SULFAMIC ACID 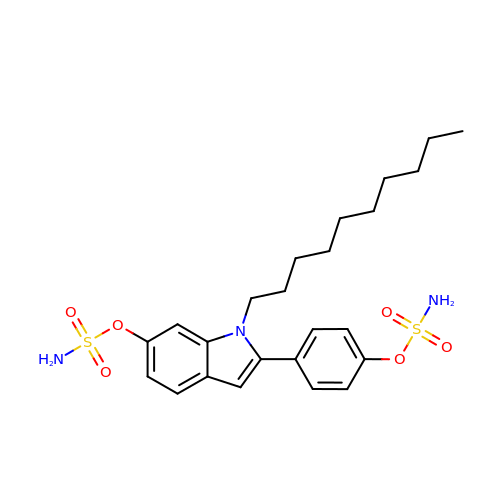1-DECYL-2-(4-SULFAMOYLOXYPHENYL)-1H-INDOL-6-YL ESTER | C24 H33 N3 O6 S2 | MXTDPQJZUVFANV-UHFFFAOYSA-N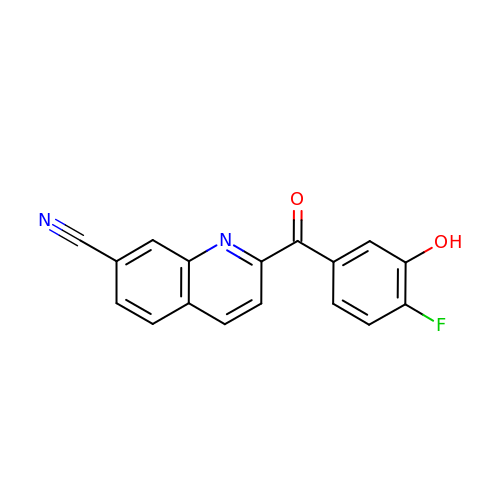2-(4-fluoranyl-3-oxidanyl-phenyl)carbonylquinoline-7-carbonitrile | C17 H9 F N2 O2 | LDOZUOMHDNDABQ-UHFFFAOYSA-N INDAN-2-AMINE | C9 H11 N | 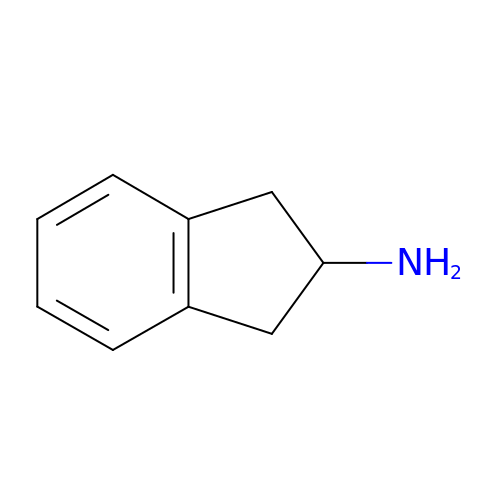LMHHFZAXSANGGM-UHFFFAOYSA-N> MADFDNLFDAAIARADETIRGYMGTSATITSGEQSGAVIRGVFDDPENISYAGQGVRVEGSSPSLF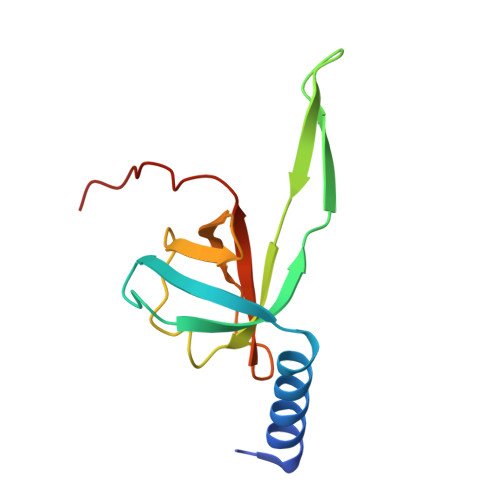VRTDEVRQLRRGDTLTIGEENFWVDRVSPDDGGSCHLWLGRGVPPAVNRRR> ARSTNTFNYATYHTLDEIYDFMDLLVAQHPELVSKLQIGRSYEGRPIYVLKFSTGGSNRPAIWIDLGIHSREWITQATGVW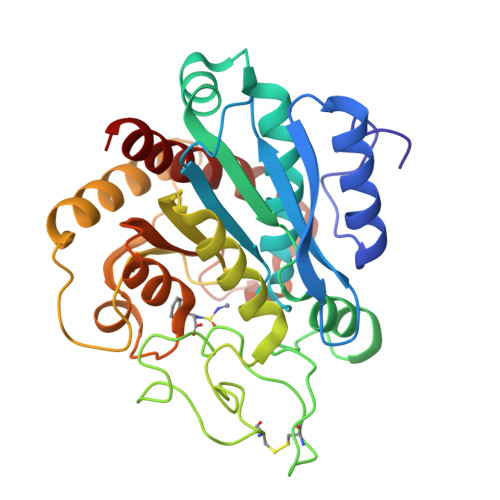FAKKFTENYGQNPSFTAILDSMDIFLEIVTNPNGFAFTHSENRLWRKTRSVTSSSLCVGVDANRNWDAGFGKAGASSSPCSETYHGKYANSEVEVKSIVDFVKNHGNFKAFLSIHSYSQLLLYPYGYTTQSIPDKTELNQVAKSAVAALKSLYGTSYKYGSIITTIYQASGGSIDWSYNQGIKYSFTFELRDTGRYGFLLPASQIIPTAQETWLGVLTIMEHTVNN>[4x]GFMKGIYSALMVPYNEDGSINEKGLREIIRYNIDKMKVDGLYVGGSTGENFMISTEEKKRVFEIAIDEAKDSVNLIAQVGSINLNEAVELGKYVTKLGYKCLSAVTPFYYKFDFSEIKDYYETIVRETGNYMIIYSIPFLTGVNMSLSQFGELFENEKIIGVKFTAGDFYLLERVRKAFPDKLIFAGFDEMLLPATVLGVDGAIGSTYNINGIRAKQIFELAKNSKIDEALKIQHTTNDLIEGILSNGLYQTIKEILKLEGVDAGYCRKPMKKISQKQIEFAKELHKKFLK

N-Acetyl-d-neuraminic acid lyase (NanA; EC 4.1.3.3) is also known as sialic acid aldolase. NanA belongs to the class I aldolase family, which is characterized by a triosephosphate isomerase (TIM)-barrel fold and by aldol condensation that proceeds through the formation of a Schiff base intermediate between a conserved lysine residue and the substrate pyruvate. Here, we report 2.32 and 1.76 Å resolution structures of N-acetylneuraminate lyase from F. nucleatum in two forms: ligand-free and with ligand bound as a pyruvate Schiff base. Sequence alignment showed that FnNanA contains conserved catalytic sites (Lys161 and Tyr133) and the conserved specific substrate (Neu5Ac) binding motif GXXGE.

The structure of ligand-free FnNanA was refined to 2.32 Å resolution. The structure has 0.35% Ramachandran outliers. The conserved Ser79 residue is in the disallowed region of the Ramachandran plot in each monomer of ligand-free FnNanA. However, electron density is well defined for Ser79. All four subunits in ligand-free FnNanA are structurally similar, and superpose with a root-mean-square deviation (r.m.s.d.) of between 0.127 and 0.169 Å for 290 Cα atoms. All four crystallographically independent monomers are very similar. Small-angle X-ray scattering data of the soluble protein also concurred that the protein was a tetramer (data not shown).>MSNKCDVVVVGGGISGMAAAKLLHDSGLNVVVLEARDRVGGRTYTLRNQKVKYVDLGGSYVGPTQNRI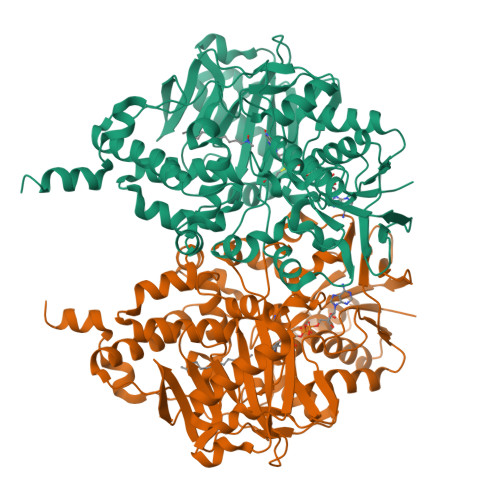LRLAKELGLETYKVNEVERLIHHVKGKSYPFRGPFPPVWNPITYLDHNNFWRTMDDMGREIPSDAPWKAPLAEEWDNMTMKELLDKLCWTESAKQLATLFVNLCVTAETHEVSALWFLWYVKQCGGTTRIISTTNGGQERKFVGGSGQVSERIMDLLGDRVKLERPVIYIDQTRENVLVETLNHEMYEAKYVISAIPPTLGMKIHFNPPLPMMRNQMITRVPLGSVIKCIVYYKEPFWRKKDYCGTMIIDGEEAPVAYTLDDTKPEGNYAAIMGFILAHKARKLARLTKEERLKKLCELYAKVLGSLEALEPVHYEEKNWCEEQYSGGCYTTYFPPGILTQYGRVLRQPVDRIYFAGTETATHWSGYMEGAVEAGERAAREILHAMGKIPEDEIWQSEPESVDVPAQPITTTFLERHLPSVPGLLRLIGLTTIFSATALGFLAHKRGLLVRV[10x]5-azanyl-6-methyl-1~{H}-pyrimidine-2,4-dione | C5 H7 N3 O2 | 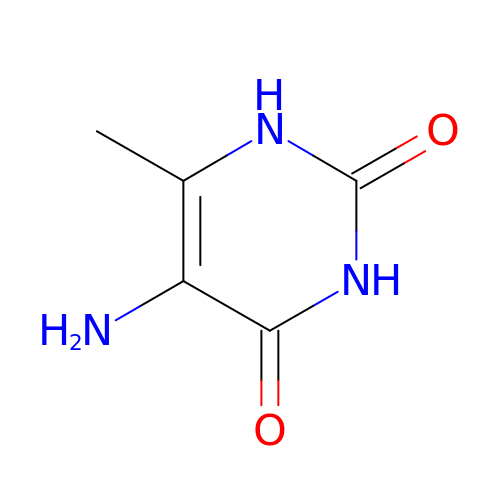FNSSATCDUXTALE-UHFFFAOYSA-N>[2x]MSKGTTSQDAPFGTLLGYAPGGVAIYSSDYSSLDPQEYEDDAVFRSYIDDEYMGHKWQAVEFARRFLFLNYGVVFTDVGMAWEIFSLRFLREVVNDNILPLQAFPNGSPRAPVAGALLIWDKGGEFKDTGHVAIITQLHGNKVRIAEQNVIHSPLPQGQQWTRELEMVVENGCYTLKDTFDDTTILGWMIQTEDTEYSLPQPEIAGELLKISGARLENKGQFDGKWLDEKDPLQNAYVQANGQVINQDPYHYYTITESAEQELIKATNELHLMYLHATDKVLKDDNLLALFDIPKILWPRLRLSWQRRRHHMITGRMDFCM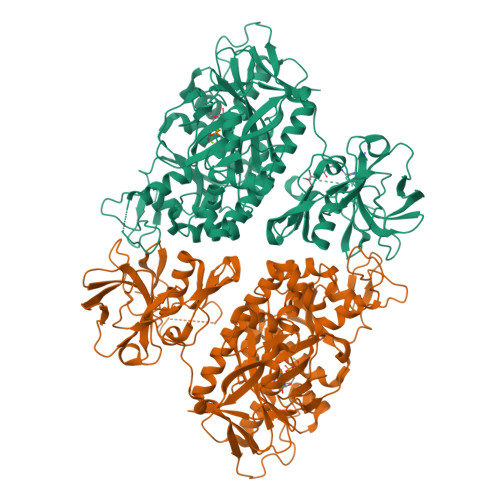DERGLKVYEYNADSASCHTEAGLILERWAEQGYKGNGFNPAEGLINELAGAWKHSRARPFVHIMQDKDIEENYHAQFMEQALHQAGFETRILRGLDELGWDAAGQLIDGEGRLVNCVWKTWAWETAFDQIREVSDREFAAVPIRTGHPQNEVRLIDVLLRPEVLVFEPLWTVIPGNKAILPILWSLFPHHRYLLDTDFTVNDELVKTGYAVKPIAGRCGSNIDLVSHHEEVLDKTSGKFAEQKNIYQQLWCLPKVDGKYIQVCTFTVGGNYGGTCLRGDESLVIKKESDIEPLIVVKK> NTGLLESQLSRHDQMLSVHDIRLADMDLRFQVLETASYNGVLIWKIRDYKRRKQEAVMGKTLSLYSQPFYTGYFGYKMCARVYLNGDGMGKGTHLSLFFVIMRGEYDALLPWPFKQKVTLMLMDQGSSRRHLGDA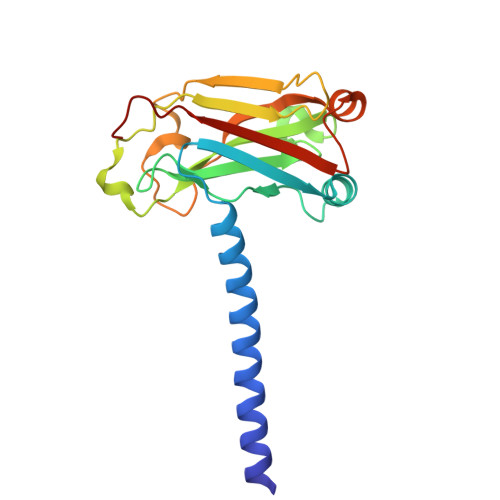FKPDPNSSSFKKPTGEMNIASGCPVFVAQTVLENGTYIKDDTIFIKVIVDTSDLPDP>ADNAPVAAQQQTQQTQKTAAAERISEQGLYAMRDVQVARLALFHGDPEKAKELTNEASALLSDDSTEWAKFAKPGKKTNLNDDQYIVINASVGISESYVATPEKEAAIKIANEKMAKGDKKGAMEELRLAGVGVMENQYLMPLKQTRNALAD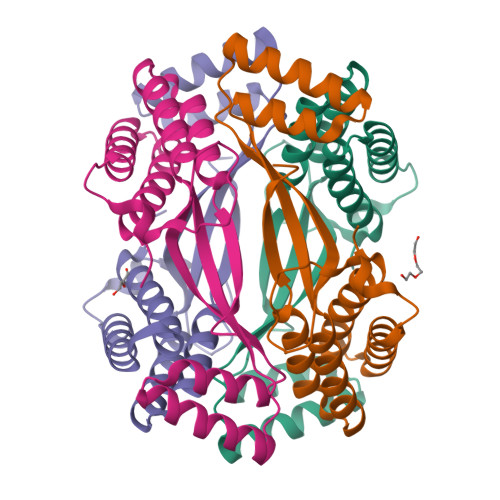AQKLLDKKQYYEANLALKGAEDGIIVDSEALFVN[8x]> MSEKPTLFSAYKMGKFNLSHRVVLAPLTRCRAINAIPNEALVEYYRQRSTAGGFLITEGTM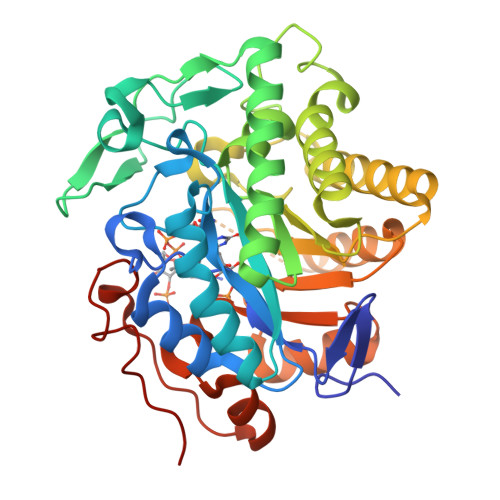ISPSSAGFPHVPGIFTKEQVEGWKKVVDAAHKEGAVIFCQLWHVGRASHQVYQPGGAAPISSTSKPISKKWEILLPDATYGTYPEPRPLAANEILEVVEDYRVAAINAIEAGFDGIEIHGAHGYLLDQFMKDGINDRTDEYGGSLENRCKFILQVVQAVSAAIGTDRVGIRISPAIDHTDAMDSDPRSLGLAVIERLNKLQFKLGSRLAYLHVTQPRYTADGHGQTEAGANGSEEEVAQLMKTWRGAYVGTFICCGGYTRELGLQAVAQGDADLVAFGRYFVSNPDLVLRLKLNAPLNRYDRATFYTHDPVVGYTDYPSLDKGSLL>[10x]GSHMGGIEVLAVRTGPDSITEIEAYLNPRMGQPQNEDFYGFSDNVTVSDDFGSDAPPWKQFPCYSTARISLPMLNQDMTSDTILMWEAISCRTEVMGVNMLTNVHSAQKRVYENDREGTGIGVEGMGYHMFAIGGEPLELQFMVFNHRATYPAEATVIKNPGASSQVFDPNLKGTLTADGVFPVEAWGPDPFKNENTRYFGQ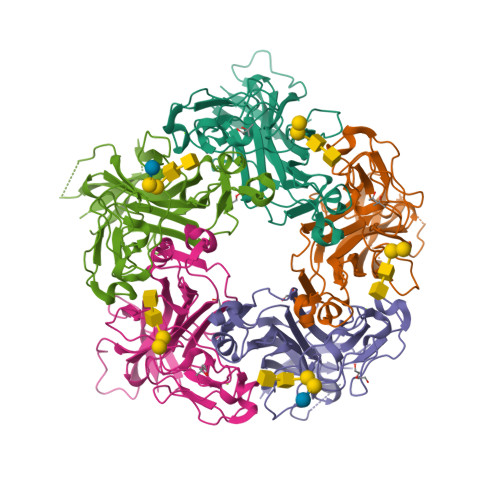YTGGTQTPPVLTFTNTQTTILLDENGVGPLCKGDGLFLSCADIVGFFTQHNKKMSFRGLPRYFRVTLRKRVVKN> NEAIECHLSDLLQQLTSVNASKPSERGLVRQEEAEDPACIPIFWVSKWVDYSDKYGLGYQLCDNSVGVLFNDSTRLILYNDGDSLQYIERDGTESYLTVSSHPNSLMKKITLLNYFRNYMSEHLLKAGANITPREGDELARLPYLRTWFRTRSAIILHLSNGTVQINFFQDHTKLILCPLMAAVTYINEKRDFQTYRLSLLEEYGCCKELASRLRYARTMVDKLLSSRSASNRLKAS

One of CSFs, Emi2 (also known as F-box only protein 43) inhibits APC/C activity by binding to APC/C-cdc20; therefore, Emi2 blocks the ubiquitin-mediated proteolysis of MPF8910. Subsequently, the phosphorylated threonines in Emi2 can be recognized by Plk1, which undergoes phosphorylation, and these phosphorylated sites serve as a recognition site for SCF, another class of ubiquitin ligases; SCF destabilizes Emi2 and activates APC/C10. In this study, one of our aim was to elucidate recognition of Emi2 by the Polo-box domain (PBD) of Plk1 using X-ray crystallography and biochemical characterization. To elucidate the detailed molecular mechanism of recognition of Emi2 by Plk1-PBD, we determined structure of the complexes of PBD domain (367–603 of Plk1) with peptides Emi2146–177 or Emi2169–177.

Furthermore, new peptidomimetics (699, 700, 701, 702, 703, 704, 705, and 706) that we developed according to the crystal structure of the complex of Plk1- PBD with Emi2, were introduced by microinjection into immature mouse oocytes, and the resulting in vitro maturation was analyzed. To identify the binding modes responsible for this strong activity, we tried to solve the structure of the complex of 103-8 with Plk1-PBD. Unfortunately, our attempts to crystallize the complex of 103-8 with Plk1-PBD were not successful. Instead, we obtained structure of the complex of PBD with peptidomimetic 702, which has a phenyl substituent that anchors bromide and methoxy groups at meta- and para-positions, respectively. The structure of the complex of Plk1-PBD with 702 is very similar to the previously solved structure of Plk1-PBD with 103-5; the latter peptidomimetic contains a hydroxy methyl group. The distance between Tyr417 and the oxygen atom of the methoxy group in 702 was found to be 4.7 Å. This finding could be attributed to the orientation of 702′s functional groups toward Tyr417. The subsequent hydrogen bonding between Tyr417 and the oxygen of the methoxy group in 702 determines the strong binding affinity.> EDPQGDAAQKTDTSHHDQDHPTFNKITPNLAEFAFSLYRQLAHQSNSTNIFFSPVSIATAFAMLSLGTKGDTHDEILEGLNFNLTEIPEAQIHEGFQELLHTLNQPDSQLQLTTGNGLFLSEGLKLVDKFLEDVKKLYHSEAFTVNFGDTEEAKKQINDYVEKGTQGKIVDLVKELDRDTVFAL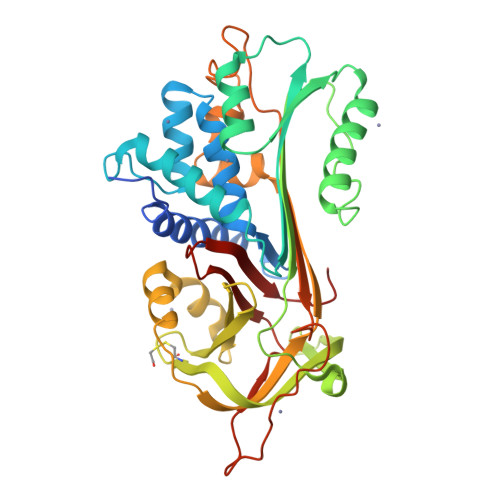VNYIFFKGKWERPFEVKDTEEEDFHVDQVTTVKVPMMKRLGMFNIQHCKKLSSWVLLMKYLGNATAIFFLPDEGKLQHLENELTHDIITKFLENEDRRSASLHLPKLSITGTYDLKSVLGQLGITKVFSNGADLSGVTEEAPLKLSKAVHKAVLTIDEKGTEAAGAMFLEAIPMSIPPEVKFNKPFVFLMIDQNTKSPLFMGKVVNPTQK PYRIDOXAL-5'-DIPHOSPHATE | C8 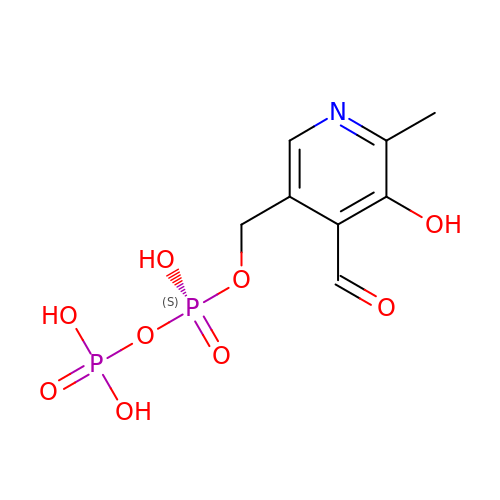H11 N O9 P2 | BLPOUZDLIYAHLN-UHFFFAOYSA-N> GEFMVSIMLLKVEDLHVYRGNREILKGVNLTVEENEIHAIIGPNGAGKSTLAYTIMG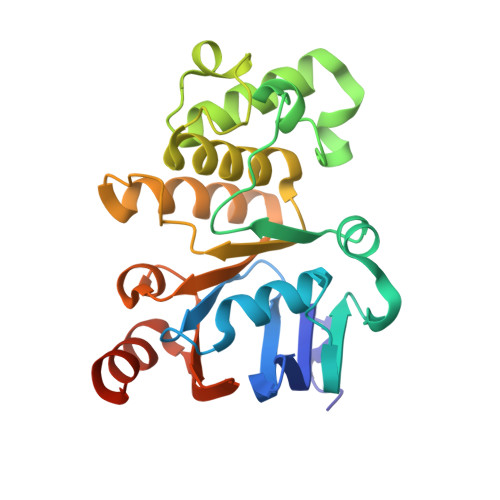ISGYKPTKGRIIFKGVDIIDKNITERARMGMTLAWQEPARFEGIKVKNYLMLGMNEKYKKDKEIAEEKIREALKLVNLDPDKYLDRYVDETLSGGERKRIELASIICMEPDLAILDEPDSGIDIVSFDEIKRVFDYLKDKGCSLLVITHREELAEHADRVSLICAGEVIKSGDPKEVGEFYKKECGKCYKKVPDGK>MAGQAFRKFLPLFDRVLVERSAAETVTKGGIMLPEKSQGKVLQATVVAVGSGSKGKGGEIQPVSVKVGDKVLLPEYGGTKVVLDDKDYFLFRDGDILGKYVD[14x];>[14x]GSAKDVKFGADARALMLQGVDLLADAVAVTMGPKGRTVIIEQSWGSPKVTKDGVTVAKSIDLKDKYKNIGAKLVQDVANNTN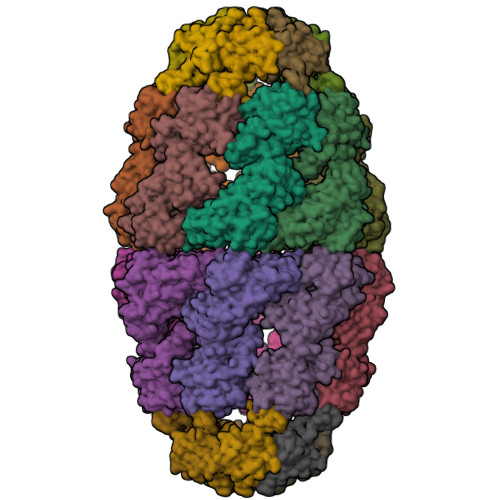EEAGDGTTTATVLARSIAKEGFEKISKGANPVEIRRGVMLAVDAVIAELKKQSKPVTTPEEIAQVATISANGDKEIGNIISDAMKKVGRKGVITVKDGKTLNDELEIIEGMKFDRGYISPYFINTSKGQKCEFQDAYVLLSEKKISSIQSIVPALEIANAHRKPLVIIAEDVDGEALSTLVLNRLKVGLQVVAVKAPGFGDNRKNQLKDMAIATGGAVFGEEGLTLNLEDVQPHDLGKVGEVIVTKDDAMLLKGKGDKAQIEKRIQEIIEQLDVTTSEYEKEKLNERLAKLSDGVAVLKVGGTSDVEVNEKKDRVTDALNATRAAVEEGIVLGGGCALLRCIPALDSLTPANEDQKIGIEIIKRTLKIPAMTIAKNAGVEGSLIVEKIMQSSSEVGYDAMAGDFVNMVEKGIIDPTKVVRTALLDAAGVASLLTTAEVVVTEIPKEEKDPGMGAMGGMGGGMGGGMF>[2x]MSRPTVVTVTETPRNPGSYEVNVERDGKMV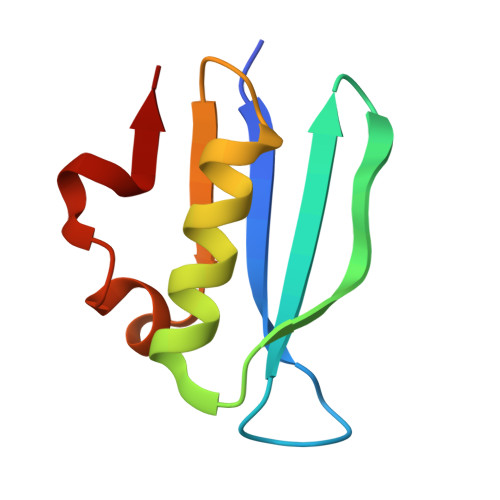VGRARAGSDPGAAAAKAMQMAMEWGSPNYVILGSNKVLAFIPEQLRVKM> G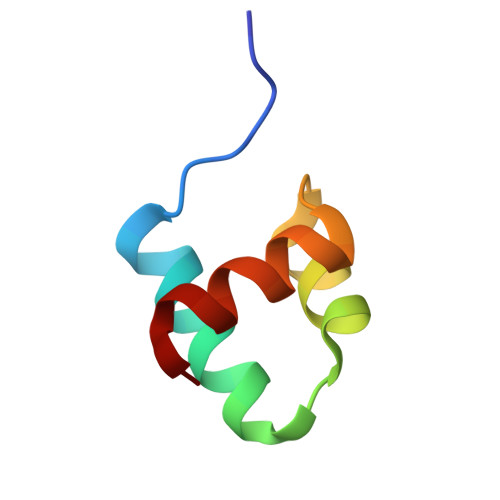AMDMSWTDERVSTLKKLWLDGLSASQIAKQLGGVTRNAVIGKVHRLGL>[12x]GSHMQASLLKVPYFVRVQGLLRICALARKIAGGHYVQMAIIKLGALTGTYVYNHLTPLRDWAHNGLRDLAVAV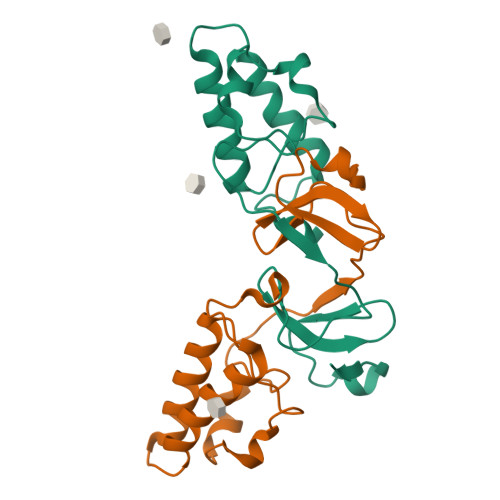EPVVFSRMETKLITWGADTAACGDIINGLPVSARRGQEILLGPADGMVSKGWRLL At present, the best structurally characterized pLGIC is the G. violaceus ligand-gated ion channel (GLIC), of prokaryotic origin. Each subunit consists of an extracellular domain (ECD), predominantly in a β-sandwich fold, and a transmembrane domain (TMD) composed of four helices, labeled M1–M4. However, the GLIC is a pH-gated channel, activated by lowering the pH, with a maximal activation at pH 4 and a pH50 around 5. We instead found that proton activation is a complex multiple loci mechanism, with the key contribution stemming from the coupling interface between the extracellular and transmembrane domain, with E35 acting as a key proton-sensing residue.

The basal principal (+) face, below Loop C, contains E82 and H127, along with a cluster of Asp/Glu residues found close to the TMD: D31, D32, and E35 from Loop 2, as well as D115 and D122 from Loop 7. Consistent with some of the previous studies of H127, H127N and Q both produce Wt-like currents. A structural analysis was performed on E26Q, E26A, E35Q, E35A, E67A, E75A, E82Q, E82A, D86A, D88N, D88A, H127N, E181A, and H277Q mutants, by solving their structure at pH 4. All structures were in the apparently open conformation. There are no significant differences, measured as 5-fold over Wt, seen in the backbone Cα residues of any of the resolved structures, with the exception of E35A and E82Q.

>[5x]GQDMVSPPPPIADEPLTVNTGIYLIESYSLDDKAETFKVNAFLSLSWKDRRLAFDPVRSGVRVKTYEPEAIWIPEIRFVNVENARDADVVDISVSPDGTVQYLERFSARVLSPLDFRRYPFDSQTLQIYLIVRSVDTRNIVLAVDLEKVGKNDDVFLTGWDIESFTAVVKPANFALEDRLESKLDYQLRISRQYFSYIPNIILPMLFILFISWTAFWSTSYEANVTLVVSTLIAHIAFNILVETNLPKTPYMTYTGAIIFMIYLFYFVAVIEVTVQHYLKVESQPARAASITRASRIAFPVVFLLANIILAFLFFGF> MNIQTTVEPTSAERAEKLQGMGCKRKRVEDIRFTQGKGNYVDDVKLPGMLFGDFVRSSHAHARIKSIDTSKAKALPGVFAVLTAADLKPLNLHYMPTLAGDVQAVLADEKVLFQNQEVAFVVAKDRYVAADAI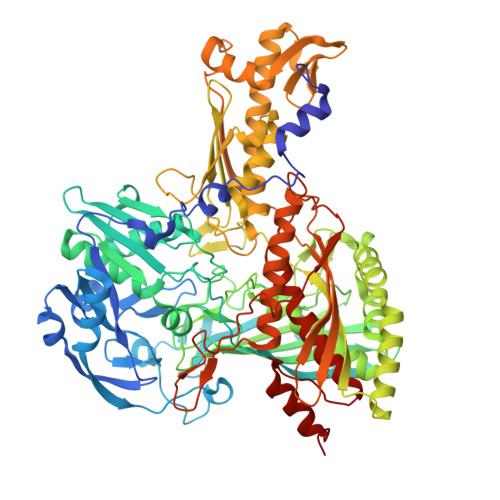ELVEVDYEPLPVLVDPFKAMEPDAPLLREDIKDKMTGAHGARKHHNHIFRWEIGDKEGTDATFAKAEVVSKDMFTYHRVHPSPLETCQCVASMDKIKGELTLWGTFQAPHVIRTVVSLISGLPEHKIHVIAPDIGGGFGNKVGAYSGYVCAVVASIVLGVPVKWVEDRMENLSTTSFARDYHMTTELAATKDGKILAMRCHVLADHGAFDACADPSKWPAGFMNICTGSYDMPVAHLAVDGVYTNKASGGVAYRCSFRVTEAVYAIERAIETLAQRLEMDSADLRIKNFIQPEQFPYMAPLGWEYDSGNYPLAMKKAMDTVGYHQLRAEQKAKQEAFKRGETREIMGIGISFFTEIVGAGPSKNCDILGVSMFDSAEIRIHPTGSVIARMGTKSQGQGHETTYAQIIATELGIPADDIMIEEGNTDTAPYGLGTYGSRSTPTAGAATAVAARKIKAKAQMIAAHMLEVHEGDLEWDVDRFRVKGLPEKFKTMKELAWASYNSPPPNLEPGLEAVNYYDPPNMTYPFGAYFCIMDIDIDTGVAKTRRFYALDDCGTRINPMIIEGQVHGGLTEAFAVAMGQEIRYDEQGNVLGASFMDFFLPTAVETPKWETDYTVTPSPHHPIGAKGVGESPHVGGVPCFSNAVNDAYAFLNAGHIQMPHDAWRLWKVGEQLGLHV>GGSHDCAKVDLENAELRRKLIRT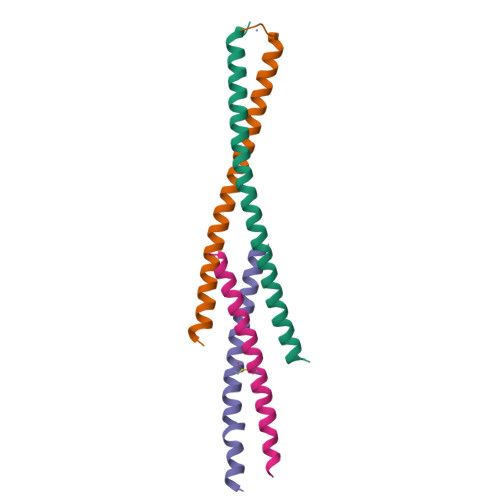KRAFEDTYEKLRMANKAKAQVEKDIKNQILKTHNVLRNVRSNMENEL[4x];>GPMDQQNSAVIGQLRLELQQARTEVETADKWRLECIDVCSVLTNRLEEEAGFLNSLLK[4x]HspB1, an abundant molecular chaperone, is prevalent in striated muscle where it is phosphorylated in response to cues including mechanical stress. Each HspB1 monomer is composed of a conserved core α-crystallin domain (ACD) flanked by a short flexible C-terminal region, which makes intra-oligomer contacts, and a longer N-terminal domain (NTD). The NTD also confers oligomeric stabilization, with phosphorylation at Ser15 and Ser78 or Ser82 causing a shift from a large polydisperse ensemble to smaller oligomeric species, including dimers. HspB1 is phosphorylated in cells and tissues in response to stretch, inducing translocation to the Z-discs and to regions of increased traction force within the cytoskeleton, suggesting that phosphorylation may trigger or modulate its interactions with mechanosensitive clients such as FLNC at these sites.

We found that a segment of the NTD just downstream of the ACD in HspB1 adopts a range of conformations and determined how they are modulated by phosphorylation to trigger oligomer dissociation. Upon refinement of the ACD, the 2Fo-Fc and difference density maps displayed a clear unmodeled feature occupying a pocket between the β3-β4 and β8-β9 loops, which lies on the side of the subunit close to the dimer interface. We were able to build peptides into this density but only accommodating subsets of the 11 possible residues, with their side-chain densities remaining poor in contrast to the ACD. An ensemble of the four peptide-bound ACDs provides the best overview of the interaction available from these data. The binding site aligns with the dynamical changes we observed by NMR. Our results reveal how the β2 strand and PPR assume heterogeneous conformations. Although predominately disordered in solution, this region is also capable of making intramonomer associations with the β3 strand and stretching to the pocket between β3-β4 and β8-β9 loops, as well as intersubunit interactions by occupying a β4-β8 groove in a neighboring dimer. While it is not clear what the relative populations of these states are in the context of the full-length HspB1, they are consistent with multiple NTD conformations contributing to maintaining sHsp assembly. Our combined data reveal that this heterogeneity is modulated by phosphorylation, resulting in changes in the stabilities of the interfaces that are likely responsible for shifting the equilibrium away from large oligomers toward smaller species. The conformational plasticity may be the primary source of the modulation in chaperone activity associated with HspB1 phosphorylation, exposing binding sites both directly through intramolecular rearrangements and indirectly by causing oligomeric dissociation.

>GVSEIRHTADRWRVSLDVNHFAPDELTVKTKDGVVEITGKHEERQDEHGYISRCFTRKYTLPPGVDPTQVSSSLSPEGTLTVEAPMP[8x];>[2x]ALSR;> LSGV;> ALSRQ2-[4-[8-oxidanylidene-2-[(~{E})-(2-oxidanylidenepyridin-3-ylidene)amino]-7~{H}-purin-9-yl]cyclohexyl]ethanenitrile 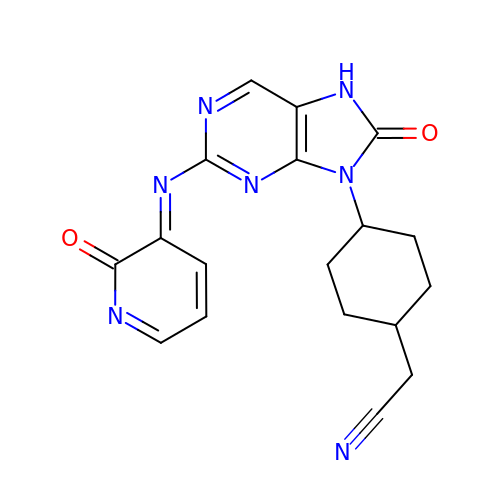| C18 H17 N7 O2 | JCBSNZZSUFHWSE-UGHOIBRWSA-N> G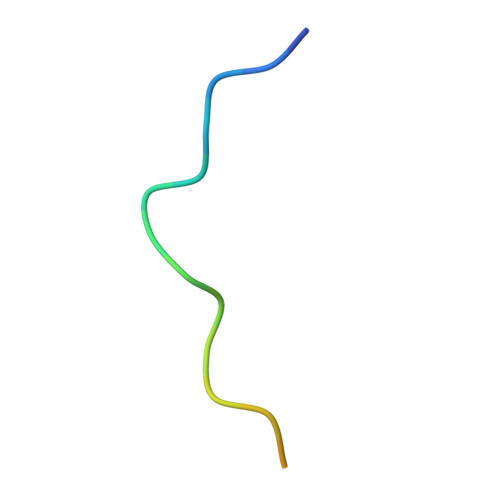PPPPPGPPPPPGPPPPPGL>MALGSRGMRIREKLEKELDPVELEVEDVSYQHAGHAAVRGSAGDDGETHFNLRIVSDAFQGKSLVKRHRLIYDLLQDELKSGLHALSIVAKTPAEV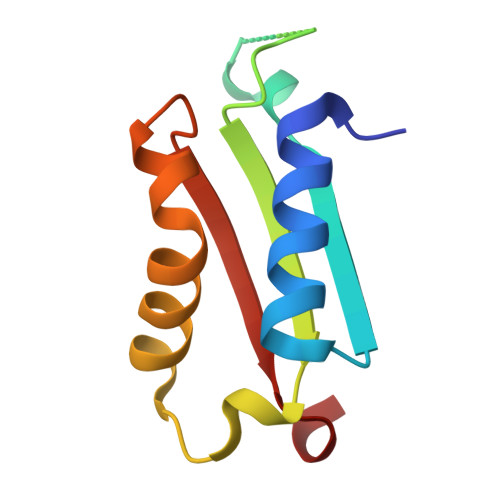[2x]>[3x]GSGTAAQPAPLTASMLASAPP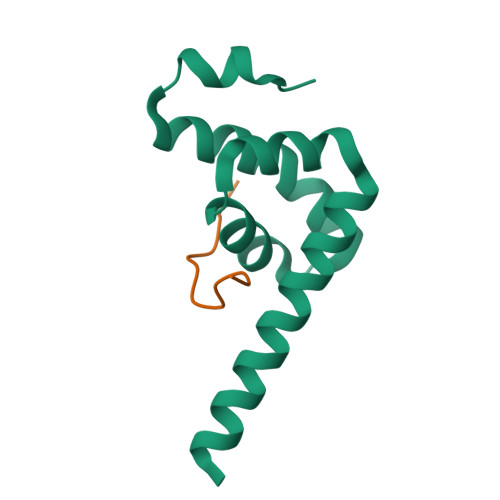QEQKQMLGERLFPLIQAMHPTLAGKITGMLLEIDNSELLHMLESPESLRSKVDEAVAVLQAHQAKEAAAAA;>HPLLNPSALEFNPSQTY[3x]> MI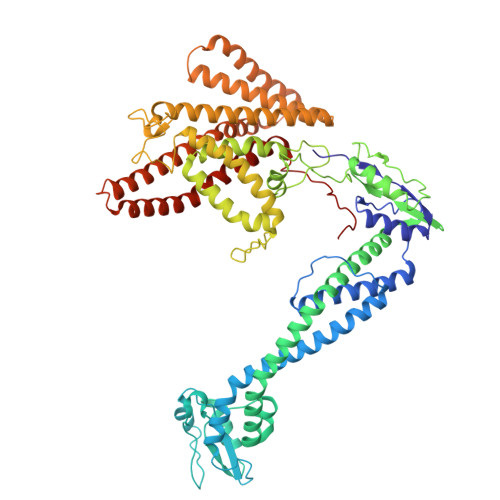APMEKLVLAGPKGRAKELLQSLQQAGVVHLETLRPEALSAYQLSPEERAELRRWEAVSAGAEHTLSLLGLEAEPARPFPEGLEAAEKALSPIQAHAEGLTRQKQELEEELALAQAYLEPLERLAALAHGLDKSPFLRVIPFLLTEKELPLVEEALRKALEDRYLLAHEAYAGGVAALVVVHRKEVDQAKAALSRAGVAELRLPGALGELPLSEAARRLKERAEAAPRELSEVRQHLAKLARESASTLQSLWTRAQDEVARLKALEELASGRFGFALLGYVPVKAKPKVEEALARHKESVVYAFEPVDEHHEADRIPVVLDNPPWAKPFELLVSFLNTPKYGTFDPTPVVPVFFPFWFGMIVGDIGYALLFYLVGRWLSGYVKRNEPLVIDLFALKLKPQVIGKLVHILNWMVFWTVVWGVIYGEFFGTFLEHLGVFGTPEHPGLIPILIHRIDTAKTANLLILLSVAFGVVLVFFGLALRAYLGLKHRHMAHFWEGVGYLGGLVGVLALAASYLGNLQAGWLQGLMYLGFGVFLLAVLMSRIWLMIPEIFTQAGHILSHIRIYAVGAAGGILAGLLTDVGFALAERLGLLGVLLGLLVAGVLHLLILLLTTLGHMLQPIRLLWVEFFTKFGFYEENGRPYRPFKSVR>[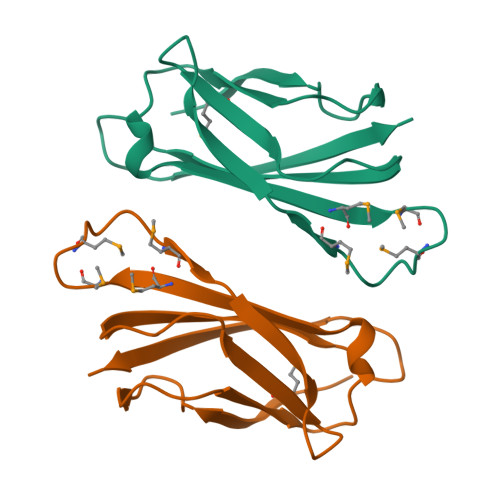2x]AHPELKSSVPQADSAVAAPEKIQLNFSENLTVKFSGAKLTMTGMKGMSSHSPMPVAAKVAPGADPKSMVIIPREPLPAGTYRVDWRAVSSDTHPITGNYTFTVK> ADAAAGAQVFAANCAACHAGGNNAVMPTKTLKADALKTYL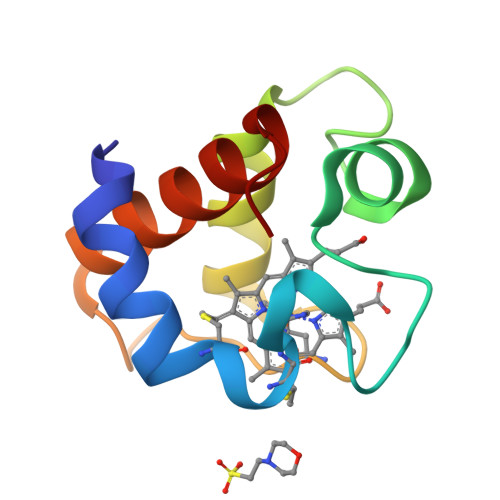AGYKDGSKSLEEAVAYQVTNGQGAMPAFGGRLSDADIANVAAYIADQAENNKW PIPERIDINE-3,4,5-TRIOL | C5 H11 N O3 | 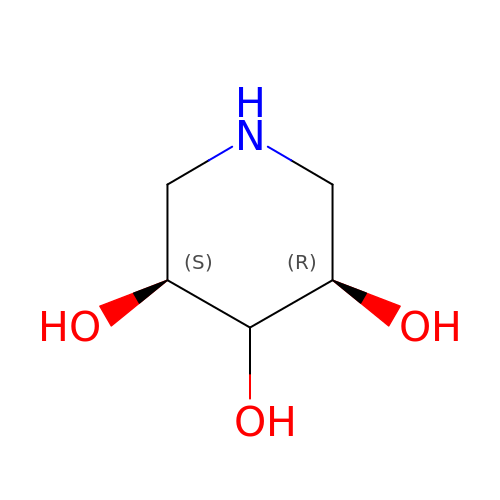RMCNETIHECSPMZ-SCDXWVJYSA-N> GAMGSGTARPGRSKVFNPYTEFPEFSRRLLKDLEKMFKTYDAGRDGFIDLMELKLMMEKLGAPQTHLGLKSMIKEVDEDFDGKLSFREFLLIFHKAAAGELQEDSGLLALAKFSEIDVALEGVRGAKNFF

EFhd1 and EFhd2 are homologous EF-hand proteins with similar structures. Although separately localized within cells, both are actin-binding proteins that modulate F-actin rearrangement through Ca2+-independent actin-binding and Ca2+-dependent actin-bundling activity. EFhd1Zn, EFhd2Zn and EFhd1Ca comprised two EF-hands, a ligand mimic (LM) helix at the C-terminus, a PR region at the N-terminus and a C-terminal linker. In addition, we determined that EFhd1 and EFhd2 bind actin independently of Ca2+ or Zn2+ and also exhibit Ca2+-dependent and Zn2+-dependent actin-bundling activity.

In the case of EFhd1Ca, CaCl2 was added to the protein solution directly to a final concentration of 4 mM. We crystallized these proteins and determined the crystal structures of EFhd1Zn, EFhd2Zn and EFhd1Ca at resolutions of 1.72, 2.60 and 2.80 Å, respectively, using molecular replacement methods [Table 1, Fig. 1(a)]. Because Zn2+ and Ca2+ have different numbers of anomalous electrons at the wavelength the EFhd1 data were collected (Zn2+ f″ = 3.9 electrons, Ca2+ f″ = 0.9 electrons), the anomalous difference map should be weaker in the Ca2+-bound state than the Zn2+-bound state. In the case of EFhd1Ca, the peak heights in the anomalous difference map were 3.4 and 2.7σ for EF-hand 1 (EF1) and EF-hand 2 (EF2), respectively. EFhd1Zn had peak heights of 23.0 and 14.0σ in the anomalous difference maps for EF1 and EF2, respectively. This suggests the metal coordinated in EFhd1Ca was Ca2+ while that coordinated in EFhd1Zn was Zn2+ [Table 3, Figs. 1(c) and 1(f)]. With EFhd1, the peak height in the anomalous difference map for the metal coordinated at the crystal-packing interface was 23.0σ in the case of EFhd1Ca. Considering both the anomalous signals and the metal coordination geometry, we deemed the metal at the interface to be Zn2+. When we superimposed the EF-hands of EFhd1Ca and EFhd1Zn and those of EFhd2Ca and EFhd2Zn, they both superimposed well (RMSD for EF1 in EFhd1Ca and EFhd1Zn = 0.100 Å for 38 Cα atoms; RMSD for EF2 in EFhd1Ca and EFhd1Zn = 0.088 Å for 35 Cα atoms; RMSD for EF1 in EFhd2Ca and EFhd2Zn = 0.157 Å for 30 Cα atoms; and RMSD for EF2 in EFhd2Ca and EFhd2Zn = 0.253 Å for 36 Cα atoms). The side-chain topologies of the EF-hand loop were similar between EFhd1Zn and EFhd1Ca and between EFhd2Zn and EFhd2Ca. This suggests the metal coordination geometries of Ca2+ and Zn2+ are similar within EFhd proteins.> 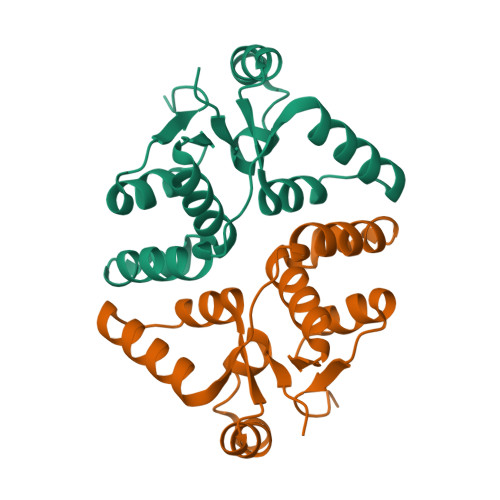MTTRYLLAKSAAYRAHLPAVRHRLEPLMERGLLARCGITDLEFGVSARSREDHRTLGTYRRDALEYVNTPDTVWVRAWEIQEALTDKGFHRSVKIPDLIIAAVAEHHGIPVMHYDQDFERIAAITRQPVEWVVAPGTALEHHHHHH> MKKCLLFLTTIALILSLSTNAFAKNTSGDLSQKQALQLALSAREHFWNTMSGHNPKVKKAVCPSGTFEYQNLQYV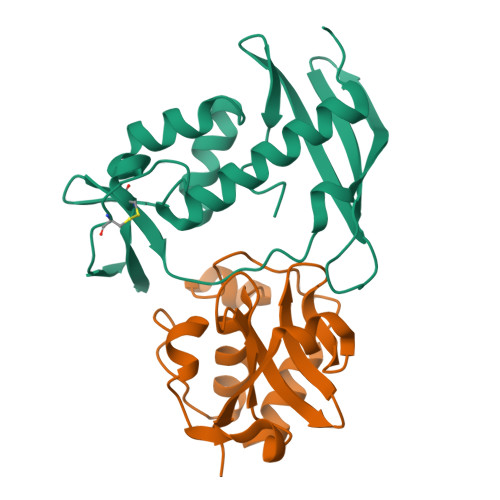YMCSDLGTKAKAVNYLTPIFTKTAIEKGFKDYHFTVSKGKLAVPIGDGDNLLNWKKSTAKLISKKGSTITYEFTVPTLDGSPSAKRKVTFVKENKKWKVNQFDAVI;> GSGGIEGAISVGSSIVGQSPYKFGGGRTQSDINNRIFDCSSFVRWAYASAGVNLGPVGGTTTDTLVGRGQAVSASEMKRGDLVFFDTYKTNGHVGIYLGNGTFLNDNTSHGVSVDSMSNPYWKAAFKGVVRRVVQ2,2-bis(oxidanyl)propanoic acid | C3 H6 O4 | 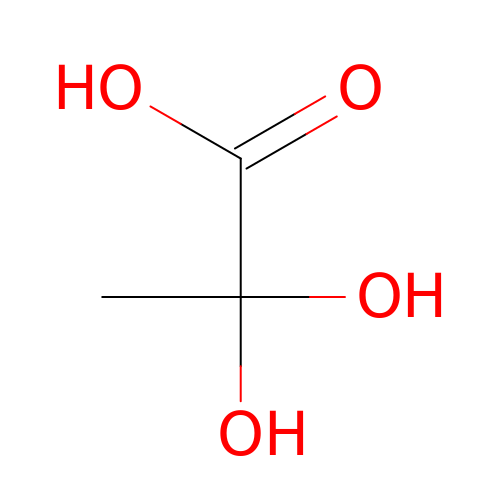HPQUMJNDQVOTAZ-UHFFFAOYSA-N>[2x]MGSSHHHHHHSMDNKTETKIEPKTGTTNFDQEALLYHQQGKPGKIEV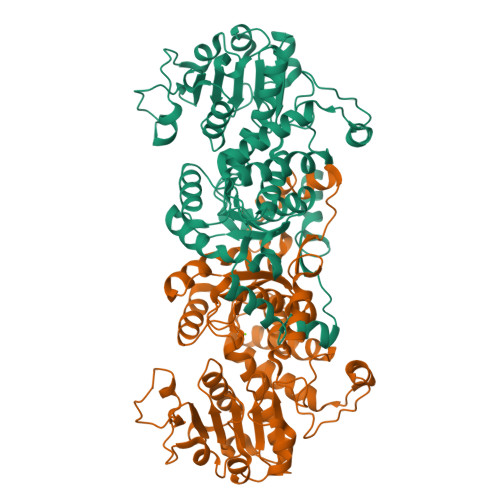ISSKPCATEKDLSLAYSPGVAAPCKAIAKDPAKVYDYTAKGNLVAVISNGTAVLGLGNIGPAAGKPVMEGKGILFKQFAGIDVFDIEVAATDVDVFCNAVRVLEPTFGGINLEDIKAPECFEIEERLKKEMNIPVFHDDQHGTAIVSGAALLNACSITNRKMETVRIVVNGAGASANSCAKIFIALGARRENIIMCDSQGVIYKGRTAGMNKYKEYFASETEARTLTEALRGADVFVGLSVAGALTPEMLKDMAKDPIIFAMANPEPEITPDKARAARPDAIIATGRSDYPNQVNNVLGFPSIFRGALDTRSTQINEEMKLAAVHALAKLAREDVPDKVSATYGGKSFKFGRDYLIPKPFDTRVLLWVAPEVAKAAMKSGVATRAIEDWDQYRESLEA> MRLEFSIYRYNPDVDDAP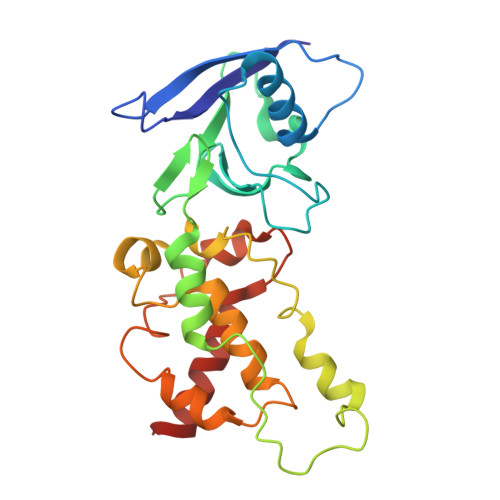RMQDYTLEADEGRDMMLLDALIQLKEKDPSLSFRRSCREGVCGSDGLNMNGKNGLACITPISALNQPGKKIVIRPLPGLPVIRDLVVDMGQFYAQYEKIKPYLLNNGQNPPAREHLQMPEQREKLDGLYECILCACCSTSCPSFWWNPDKFIGPAGLLAAYRFLIDSRDTETDSRLDGLSDAFSVFRCHSIMNCVSVCPKGLNPTRAIGHIKSMLLQRNA>[2x]GSHMPYAAVNGTELHYRIDGERHGNAPWIVLSNSLGTDLSMWAPQVAALSKHFRVLRYDTRGHGHSEAPKGPYTIEQLTGDVLGLMDTLKIARANFCGLSMGGLTGVALAARHADRIERVALCNTAARIGSPEVWVPRAVKARTEGMHALADAVLPRWFTADYMEREPVVLA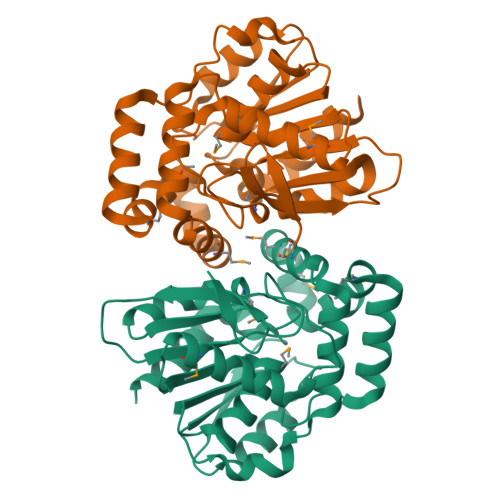MIRDVFVHTDKEGYASNCEAIDAADLRPEAPGIKVPALVISGTHDLAATPAQGRELAQAIAGARYVELDASHISNIERADAFTKTVVDFLTEQK> MDMLSPVVREAEVSRAARRQSSNRKNPADESWSNATPTRGPSSRTTGQTLFRQHMTPQTWNSSRPPDVSAILGTVGRSPRLLQTPGRLANLSMMSNPDDSVWTTTFSPGRTGMYTTLDSPSFTEDITLSAVMLQEEDPGEAATMSMYPDFLKSFLEHPSSAVFELIEQYEATCNTQITLLKKIVKRVTPGQQKFSKTASILWLLQQEMVTWRLIAALYRDRIQSALEEENMFEIAAPNASEKTIVDKLFQRDTLVRQSQLVVDWLESIAKDEVGDFSDNIEYYAKSVYWENTLHTLKQRSMLSLGSSRPLVSELDPDAPIRQKLPLDDLDREDDIRLLKYLFTLIRAGMTDEAQR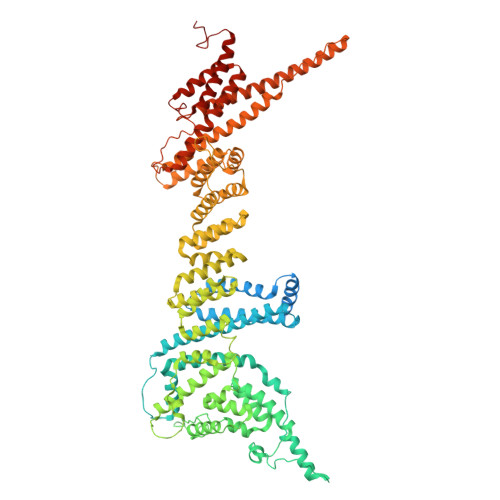LCKRCGQAWRAATLEGWKLYHDANINGGTELQAVEGNPYRCVWKTCCWRMAEDEQFNKYERAIYATLSGNLKQLLPVCESWEDTVWAHFKVMVDSLVEQEIRASIISFNEANELPREYLEANWTLDSVFEELQATDKKRVLEENREHYHIIQKFVILADVDGLMDEFSEWLSNGKNLLLGHLLRFMTHLLLFFRTLGLQAKEEVSVEVLKTYIQRLINEKQIELIAFYVSHLPQELAISQYAVFLENITDPDQRQRCLELAKEAGLDVASITKTVVENTRKKDAGEFAHHDFAPALDSGTSEEDRAKIDVIDWLVFDPAQRAEALKQSNAIMRKFLASKKHEAAKEVFAKIPQDSIAEIYSQWEEQAMDSALPAEDDNAIREHLCIRAYLESHEAFNEWFKHINSPPQKPTLVGQASFTEKVAHEHKEKKYEMDFGIWKGHLDALTSDVKEKIYNVLLFVDGGWMVDVREDTEEDPERSHQMVLLRRLCLPMMCFLLHTVLHNTKQYKDCLRLADIVSSENQKLYTVFSKTEMRNLLQKLRESSLMLLDLQLDPLGYEIQS> MAPITAYSQQTRGLLGCIITSLTGRDRNQVEGEVQVVSTATQSFLATCVNGVCWTVYHGAGSKTLAGPKGPITQMYTNVDQDLVGWQAPPGARSLTPCTCGSSDLYLVTRHADVIPVRRRGDSRGSLLSPRPVSYLKGSSGGPLLCPSGHAVGIF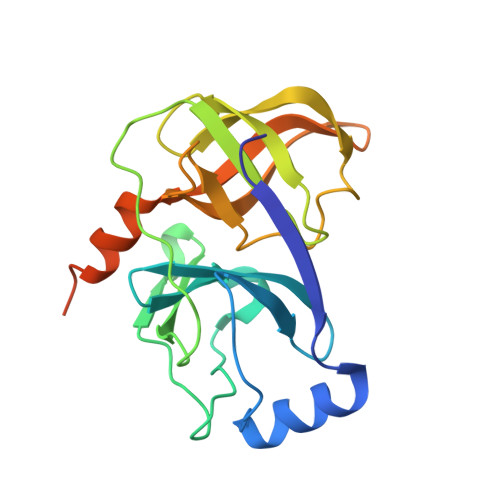RAAVCTRGVAKAVDFVPVESMETTMRASKKKKKGSVVIVGRIILSGRK2-(1-benzothiophen-7-yl)-4-[1-(piperidin-4-yl)-1H-pyrazol-4-yl]furo[2,3-c]pyridin-7-amine | C23 H21 N5 O S | 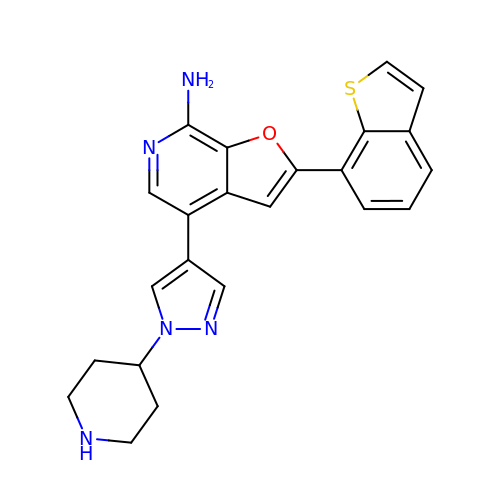HYMAZAOGZLVDSM-UHFFFAOYSA-N> QGPAMAGN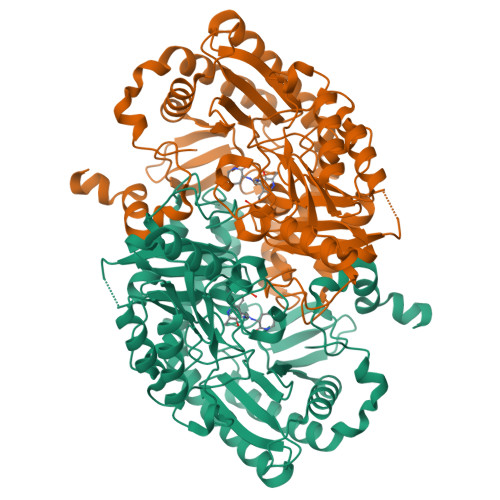LYGRDGAAIGSLQKLRFFPLAVAGGQGARLVEEDGRELIDLSGAWGAASLGYGHPAIIEAVSRAAANPAGASILSASNAPAVALAERLTASFPGRGTHKVWFGHSGSDANEAAYRAITRATGRTGVIAFIGAYHGCTVGSMAFSGHSVQADAAKADGLILLPYPDPYRPYQDDPTGDAVLALLKERLAAVPAGSIAAAFIEPIQSAGGLIVPPDGFLRKFADICRAHGISVVCDEVKVGLARSGRLHCFEHEGFVPDILVLGKGLGGGLPLSAVIAPAEILDCASAFAMQTLHGNPVCAAAGLAVLETIEAENLTTAAERKGKLLREGLARLAERHELIGDIRGRGLACGVELVRNRQSREPARAETAKLIYRAYELGLVLYYVGMNGNVLEMTPPLTMTEDEVRHAVNLLDQAFTELSTVSDTLVSQFAGW> MEMTSAFTLNVRLDNIAVITIDVPGEKMNTLKAEFASQVRAIIKQLRENKELRGVVFVSAKPDNFIAGADINMIGNCKTAQEAEALARQGQQLMAEIHALPIQVIAAIHGACLGGGLELALACHGRVCTDDPKTVLGLPEVQLGLLPGSGGTQRLPRLIGVSTALEMILTGKQLRAKQALKLGLVDDVVPHSILLEAAVELAKKERPSSRPLPVRERILAGPLGRALLFKMVGKKTEHKTQGNYPATERILEVVETGLAQGTSSGYDAEARAFGELAMTPQSQALRSIFFASTDVKKDPGSDAPPAPLNSVGILGGGLMGGGIAYVTACKAGIPVRIKDINPQGINHALKYSWDQLEGKVRRRHLKASERDKQLALISGTTDYRGFAHRDLIIEAVFENLELKQQMVAEVEQNCAAHTIFASNTSSLPIGDIAAHATRPEQVIGLHFFSPVEKMPLVEIIPHAGTSAQTIATTVKLAKKQGKTPIVVRDKAGFYVNRILAPYINEAIRMLTQGERVEHIDAALVKFGFPVGPIQLLDEVGIDTGTKIIPVLEAAYGERFSAPANVVSSILNDDRKGRKNGRGFYLYGQKGRKSKKQVDPAIYPLIGTQGQGRISAPQVAERCVMLMLNEAVRCVDEQVIRS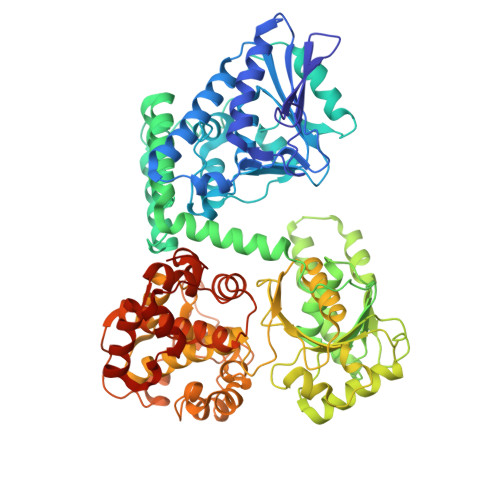VRDGDIGAVFGIGFPPFLGGPFRYIDSLGAGEVVAIMQRLATQYGSRFTPCERLVEMGARGESFWKTTATDLQ> MGLNVASVKSYVSSALTTTLFGSGVGEREVGKLTSIIMNKMLFAQGWQFSVEVDGLEGADFFAKDITYHDYSIEYE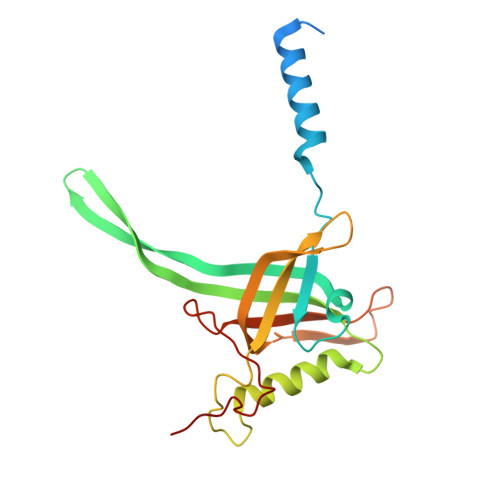TIKIGGGNILQPTERSPGQITMMVRDTVDGLVLDWFKTAKSRVINPDGTGNIPSQYLLNVRIYRLLSSGLTKLENEMTVFPVTTGDVTYARDQVTEFKSFPMTFALHSTFNQSSSSLASLLGFSFSL> SSGSKSSNSSAKKSAGKPQQGGDLVVGSIGEPTLF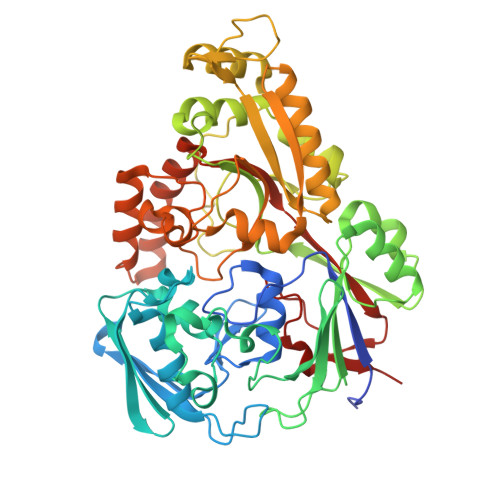NSLYSTDDASTDIENMLYSFLTKTDEKLNVKLSLAESIKELDGGLAYDVKIKKGVKFHDGKELTADDVVFTYSVPLSKDYKGERGSTYEMLKSVEKKGDYEVLFKLKYKDGNFYNNALDSTAILPKHILGNVPIADLEENEFNRKKPIGSGPFKFKEWKQGQYIKLEANDDYFEGRPYLDTVTYKVIPDANAAEAQLQAGDINFFNVPATDYKTAEKFNNLKIVTDLALSYVYIGWNEKNELFKDKKVRQALTTALDRESIVSQVLDGDGEVAYIPESPLSWNYPKDIDVPKFEYNEKKAKQMLAEAGWKDTNGDGILDKDGKKFSFTLKTNQGNKVREDIAVVVQEQLKKIGIEVKTQIVEWSALVEQMNPPNWDFDAMVMGWSLSTFPDQYDIFHSSQIKKGLNYVWYKNAEADKLMKDAKSISDRKQYSKEYEQIYQKIAEDQPYTFLYYPNNHMAMPENLEGYKYHPKRDLYNIEKWWLAK Leucine aminopeptidase (LAP) is found in all kingdoms of life and catalyzes the metal-dependent hydrolysis of the N-terminal amino acid residue of peptide or amino acyl substrates. We report here the X-ray structures of three kinetoplastid acidic LAPs (LAP-As from Trypanosoma brucei, Trypanosoma cruzi, and Leishmania major) which were solved in the metal-free and unliganded forms, as well as in a number of ligand complexes, providing insight into ligand binding, metal ion requirements, and oligomeric state. LAPs of the M17 family of aminopeptidases are bilobal proteins with a highly conserved C-terminal domain harboring the aminopeptidase activity. They form homohexamers of approximately 330 kDa with the active sites facing a central cavity separated from the bulk solvent but accessible through solvent channels.

LmLAP-A crystallized under many different conditions, forming hexagonal plate-like crystals, one of which, grown in the presence of actinonin, diffracted to 2.5 Å and was in space group P321. Structural differences in LmLAP-A compared to TbLAP-A and TcLAP-A are mostly located in the loop regions. The secondary structure elements and their positions in LmLAP-A are nearly identical to those in TbLAP-A, with the exceptions of β1, β3, and β4, which are shortened, and α2, which is replaced by a loop. The N terminus of LmLAP-A is extended and forms a loop before the start of the α1 helix. For both the TbLAP-A and LmLAP-A complexes, the electron density was sufficient to model the ligand, albeit with less than 100% occupancy. Actinonin in LmLAP-A and TbLAP-A is coordinated by the Mn2+ ions and hydrogen bonds. In both structures, the two Mn2+ atoms coordinate the O-2 and O-4 oxygen atoms of the ligand. In LmLAP-A, the side chains of K299, D304, K311, and D389 form hydrogen bonds with O-2 and O-4, and the main-chain oxygen of L420 and the main-chain nitrogen of G422 form hydrogen bonds with N-1 and O-13, respectively. The N-14 atom of actinonin coordinates a water molecule. Superposition of the active sites including the actinonin molecules reveals the high similarity of the conformations actinonin adopts, with the only difference being in the hydroxymethyl-pyrrolidine moiety, which forms a hydrogen bond in TbLAP-A but not in LmLAP-A, where it is bent away from the corresponding residue (A424).

> MSAMKRPRSNSIVEETAVSAYVQTCTNFKSNVTFTDISKVSCVAYHVLLVGALEQLRDNSLKSVLFYCPAVAEALQRVKAGSTVKTLAEVPGRKGYTEVMVTALPATTSRTNCPYRADSMSEAVAAACGSVEEGEVLDVYVCAPAGSETAVANAVARAAPHSYTAKAGQATKAYMKQAMSLNVVMSSRAAFTQELVRGKSVCVAELEAICTSVQLCQRLVDTPPCMLDTVVYAEIAAAYAAELGVDMTVIKGDELREKGYGGIYAVGKCAQYPAHLVTLRYRNPNAAEGAKNIAMVGKGIVYDCGGLALKPAAHMTNMKTDMGGSAGVFCAFIAVVRSMKMQRTHFSHIANISVTLCLAENAIGPHSYRNDDVVVMKSGKSVEVMNTDAEGRIVLGDGVYYATGEQDFVPDVLIDMATLTGAQGVATGSKHAGVYASDAEAEKDMISAGLQSGDLCYPVLYCPEYHEEVYKSPCADMRNIANSSSSAGSSCGGYFVEQHLSERFRGPFVHVDMAYPTSNTAGATGYGVTLVFEFLRQH>CGGCCG[2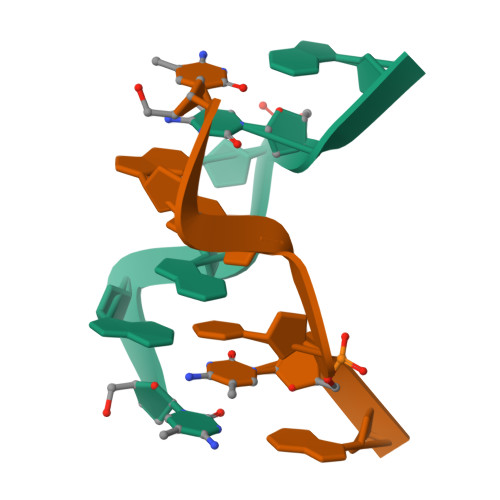x]> GEFEEPDFTALCQKLKIPDHVRERAWLTWEKVSSVDGVLGGYIQKKKELWGICIFIAAVDLDEMSFTFTELQKNIEISVHKFFNLLKEIDTSTKVDNAMSRLLKKYDVLFALFSKLERTCELIYLTQPSSSISTEINSALVLKVSWITFLLAKGEVLQMEDDLVISFQLMLCVLDYFIKLSPPMLLKEPYKTAVIENDTRIIEVLCKEHECNIDEVANVAFKNFIPFMNSLGLV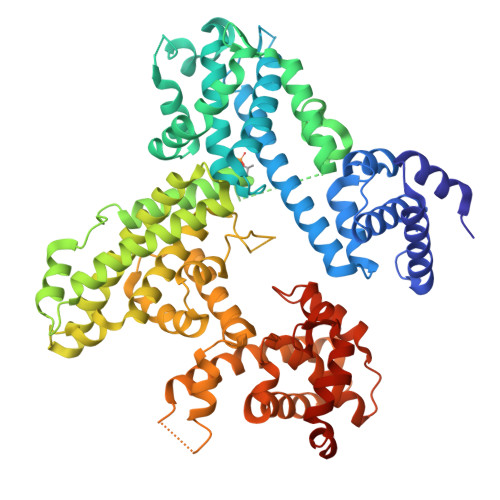TSNGLPEVENLSKRYEEIYLKNKDLDARLFLDHDKTLQTDSIDSFETQRTPRKSNLDEEVNVIPPHTPVRTVMNTIQQLMMILNSASDQPSENLISYFNNCTVNPKESILKRVKDIGYIFKEKFAKAVGQGCVEIGSQRYKLGVRLYYRVMESMLKSEEERLSIQNFSKLLNDNIFHMSLLACALEVVMATYSRSTSQNLDSGTDLSFPWILNVLNLKAFDFYKVIESFIKAEGNLTREMIKHLERCEHRIMESLAWLSDSPLFDLIKQSKDREGPLKSTSLSLFYKKVYRLAYLRLNTLCERLLSEHPELEHIIWTLFQHTLQNEYELMRDRHLDQIMMCSMYGICKVKNIDLKFKIIVTAYKDLPHAVQETFKRVLIKEEEYDSIIVFYNSVFMQRLKTNILQYASTRPPTLAPIPHIPR Roundabout (Robo) receptors provide an essential repulsive cue in neuronal development following Slit ligand binding. The Drosophila and vertebrate Robo1-3 are most similar, containing five immunoglobulin (Ig) and three fibronectin (Fn) domains in their extracellular region. Here we present the crystal structure of Robo1 Ig1-4 and Robo1 Ig5, together with a negative stain electron microscopy reconstruction of the Robo1 ectodomain. These results show how the Robo1 ectodomain is arranged as compact dimers, mainly mediated by the central Ig domains, which can further interact in a “back-to-back” fashion to generate a tetrameric assembly.

An inspection of the potential N-glycosylation site at N463 reveals no additional density. All five Robo1 Ig domains are very similar, the main conformational difference occurring in the βC-βD loop region. Interestingly, the βE-βF loop region in Ig1, which contributes two sequence conserved basic residues (K137 and R136) required for heparin binding (Fukuhara et al., 2008), is longer than those observed in the other four Ig domains. Rigid body modeling of the Robo1 Ig1-5 construct by adding the Ig5 domain determined allowed us to fit the corresponding SAXS data rather well (χ2 = 1.3), yielding a model similar to the previously computed ab initio shape. The Robo1 Ig1-5 has a Dmax of ∼200 Å, indicating that Robo1 Ig1-5 does not adopt an extended conformation and consistent with the EM map having a largest dimension of ∼190 Å. This constraint, including an eight-amino acid linker region between Ig4 and Ig5, provided the basis to model Ig5 in a looping back orientation. The flexible linker regions between Ig4-5 and Ig5-Fn1 enable these domains to loop back toward the N terminus before extending down to the cell surface via Fn2-3.

> PPVIRQGPVNQTVAVDGTFVLSCVATGSPVPTILWRKDGVLVSTQDSRIKQLENGVLQIRYAKLGDTGRYTCIASTPSGEATWSAYIEVQAG>GSHMVKLKVEDLEMDKIAPLAPEVSLKMAWNIMRDKNLKSIPVADGNNHLLGMLSTSNITATYMDIWDSNILAKSATSLDNILDTLSAEAQNINEERKVFPGKVVVAAMQAESLKEFISEGDIAIAGDRAEIQAELIELKVS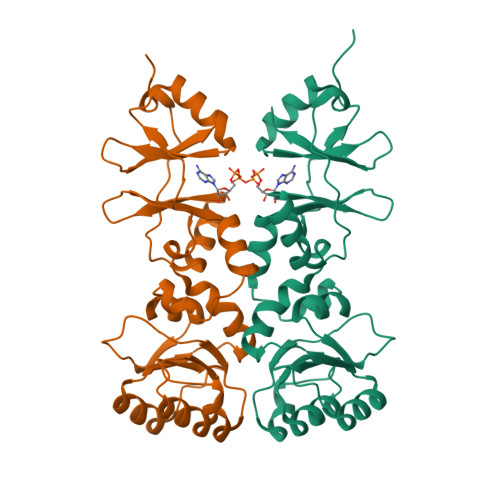LLIVTGGHTPSKEIIELAKKNNITVITTPHDSFTASRLIVQSLPVDYVMTKDNLVAVSTDDLVEDVKVTMSETRYSNYPVIDENNKVVGSIARFHLISTHKKK[2x]> MIKATYSSAKDFYSLLSGLLKVTDEIILNFTEDSIF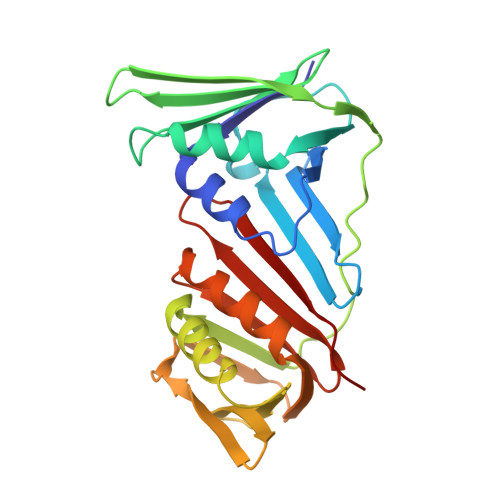SRYLTDDKVLMVIFKIPKEYLEDYTIDKPLGIKININDLKKILGKAKSKSATVTLEETEAGLKVTVRDEKTGTRSNIYIKGEKTSIDQLTEPKVNLSVTFTTDGDVLKDIARDLSLVGEEVEISADENTVTLSTEEAGRTYKSLLKQDKPLKSLNVESPSKAVYSIEVLKDVFKVTSISQNVTVGFGNNIPMKIEVPTDSGGQLIFWIAPRL N-{(1S,2S)-2-[(4aS,7aR)-2-amino-4a,5-dihydro-4H-furo[3,4-d][1,3]thiazin-7a(7H)-yl]cyclopropyl}-5-fluoropyridine-2-carboxamide | C15 H17 F N4 O2 S | 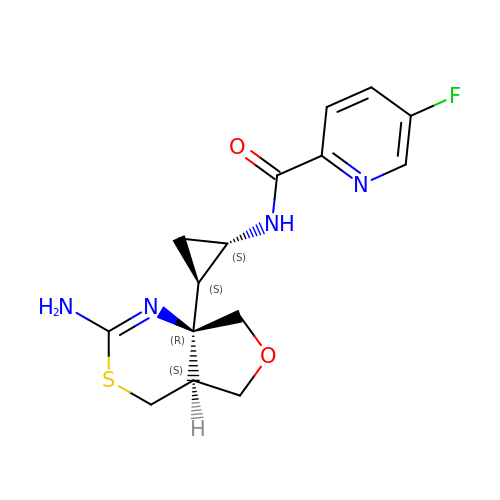OWWIYTVWTQBRDL-FGAILIKWSA-N> MYKATVIIKLKKGVLNPEGRTIQRALNFLGFNNVKEVQTYKMI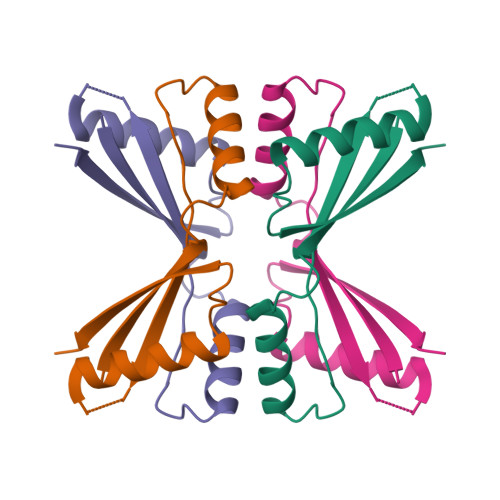DIIMEGENEEKVKEEVEEMCKKLLANPVIHDYEIKVEKIE>GGADQKGPVFLKEPTNRIDFSNSTGAEIECKASGNPMPEIIWIRSDGTAVGDVPGLRQISSDGKLVFPPFRAEDYRQEVHAQVYACLARNQFGSIISRDVHVRAVVNQFYGADILMEYVIRGNAAVLKCSIPSFVADFVRVESWIDEEGTELRPSENYDGKYLVLPSGELHIREVGPEDGYKSYQCRTKHRLTGETRLSATKGRLVITEPVGSVRPKVNPQDKHQFIDVELASSYSLLCMAQSYPTPSFRWYKFIEGTTRKQAVVLNDRVKQVSGTLIIKDAVVEDSGKYLCVVNNSVGGESVETVLTVTAPLSAKIDPPTQTVDFGRPAVFTCQYTGNPIKTVSWMKDGKAIGHSEPVLRIES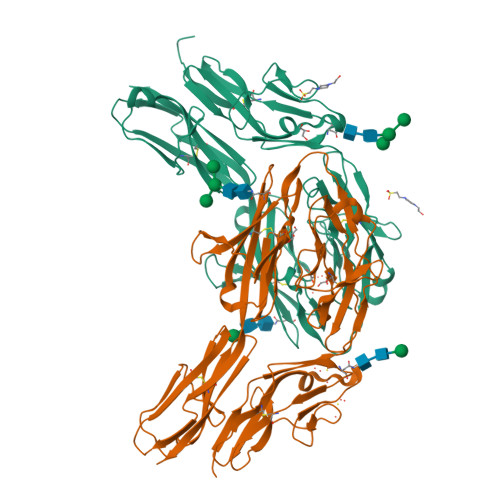VKKEDKGMYQCFVRNDQESAEASAELKLGG[2x]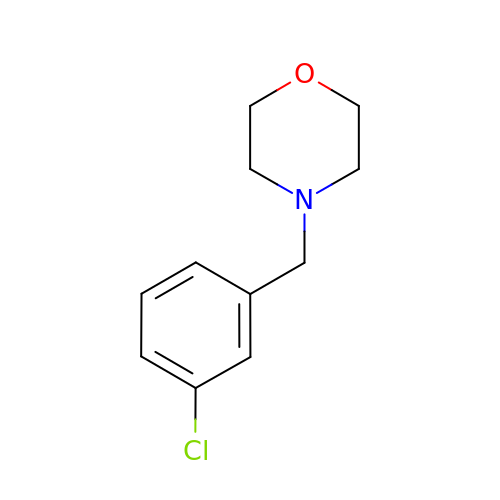4-[(3-chlorophenyl)methyl]morpholine | C11 H14 Cl N O | NWMZWMSJQLEJTG-UHFFFAOYSA-N11,15-dimethyl-6-(oxan-4-yloxy)-8-oxa-2,11,15,19,21,23-hexazatetracyclo[15.6.1.13,7.020,24]pentacosa-1(23),3(25),4,6,17,20(24),21-heptaen-10-one   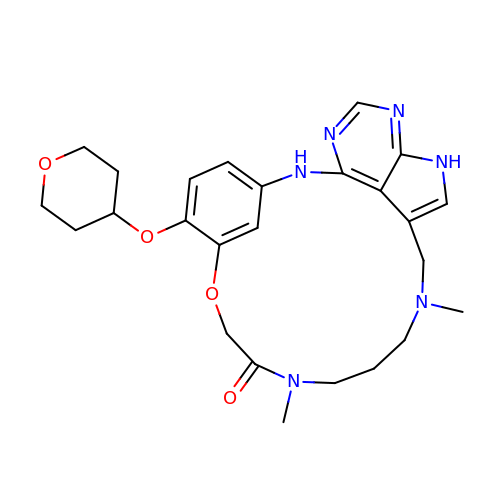| C25 H32 N6 O4 | QMBXNOSHZHHYKG-UHFFFAOYSA-N>ETGSAQQLNEDLRLHLLLNTSVTCNDGSPAGYYLKESRGSRRWLLFLEGGWYCFNRENCDSRYDTMRRLMSSRDWPRTRTGTGILSSQPEENPYWWNANMVFIPYCSSDVWSGASSKSEKNEYAFMGALIIQEVVRELLGRGLSGAKVLLLAGSSAGGTGVLLNVDRVAEQLEKLGYPAIQVRGLADSGWFLDNKQYRHTDCVDTITCAPTEAIRRGIRYWNGVVPERCRRQFQEGEEWNCFFGYKVYPTLRSPVFVVQWLFDEAQLTVDNVHLTGQPVQEGLRLYIQNLGRELRHTLKDVPA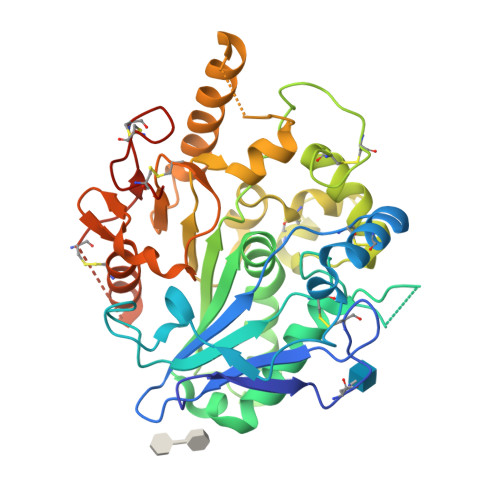SFAPACLSHEIIIRSHWTDVQVKGTSLPRALHCWDRSLHDSHKASKTPLKGCPVHLVDSCPWPHCNPSCPTGTKHHHHHH[2x]> HMASMKKKGS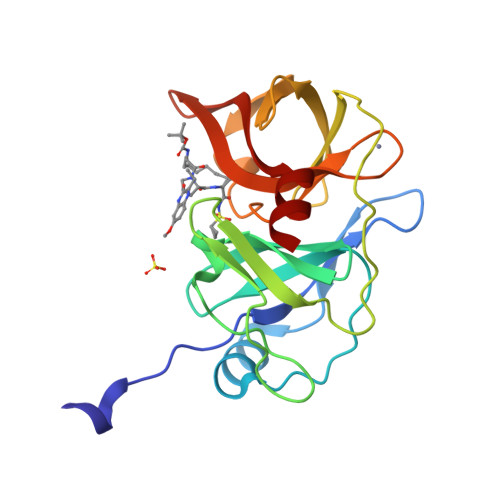VVIVGRINLSGDTAYAQQTRGEEGCQETSQTGRDKNQVEGEVQIVSTATQTFLATSINGVLWTVYHGAGTRTIASPKGPVTQMYTNVDKDLVGWQAPQGSRSLTPCTCGSSDLYLVTRHADVIPVRRRGDSRGSLLSPRPISYLKGSAGGPLLCPAGHAVGIFRTAVSTRGVAKAVDFIPVESLETTM>[4x]MNEALDDIDRILVRELAADGRATLSELATRAGLSV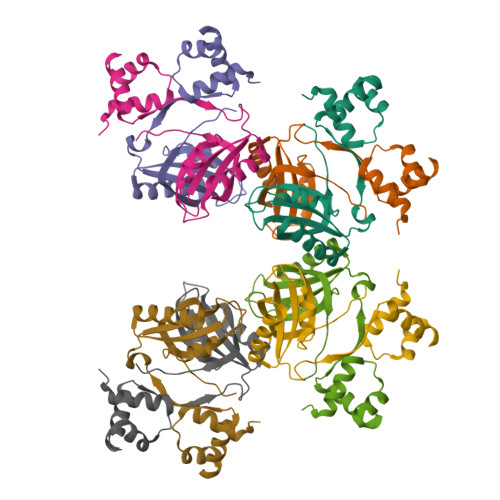SAVQSRVRRLESRGVVQGYSARINPEAVGHLLSAFVAITPLDPSQPDDAPARLEHIEEVESCYSVATEESYVLLVRVASARALEDLLQRIRTTANVRTRSTIILNTFYSDRQHIP> MSGSNSTANGANSTASGDNSTASGTNASATGENSTATGTDSTASGSNSTANGTNSTASGNNSTASGTNASATGENSTATGTDSAASGTNSTANGTNSTASGDNSTASGTNASATGENSTATGTASTASGSNSTANGANSTASGAGATATGENAAATGAGATATGNNASASGTSSTAGGANAIASGENSTTNGANSTASGNGSSAFGESAAAAGDGSTALGANAVASGVGSVATGAGSVASGANSSAYGTGSNA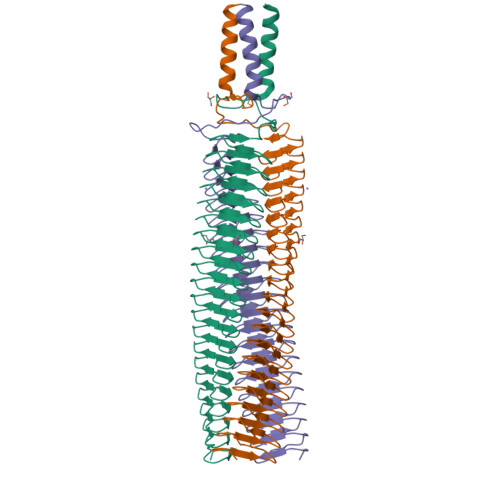TGAGSVAIGQGATASGSNSVALGTGSVASEDNTVSVGSAGSERRITNVAAGVNATDAVNVGQMKQIEDKIEEILSKIYXXXXXXXXXXXXXXXXXXXX>[2x]MKKHHISMINIPAYGHVNPTLALVEKLCEKGHRVTYATTEEFAPAVQQAGGEALIYHTSLNIDPKQIREMMEKNDATLSLLKESLSILPQLEELYK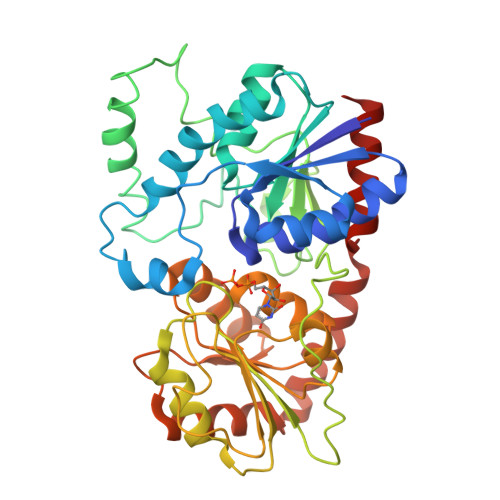DDQPDLIIYDFVALAGKLFADKLNVPVIKLCSSYAQNESFQLGNEDMLKKIKEAEAEFKAYLEQEQLPAVSFEQLAVPEALNIVFMPKSFQIQHETFDDRFCFVGPSLGKRTEQESLLIDKGDRPLMLISLGTAFNAWPEFYKMCIDAFRDSSWQVIMSVGKSIDPESLDDTPANFTIRQSVPQLEVLAKADLFISHGGMNSTMEAMNAGVPLVVIPQMYEQELTAKRVDELGLGVYLQREEVTVSKLQEAVQAVSGDQELLSRVKSMQKDVKEAGGAERAAAEIEAFMKKSAVPQ> MKNAIVIGAGIGGLAAALRLRHQGYSVTIFEKNDYAGGKLHAIEKDGYRFDLGPSLFTLPHLVENLFALFPEEIIDFGYKSKAISFHYFWDDGTLFKASTDSSQFIEDASKVFKEEKSTIKKYLAKSKSKYELTKSLFLEKSLHKATTYFSLDTVKAIVHAPFLGLNNTLNDENSKF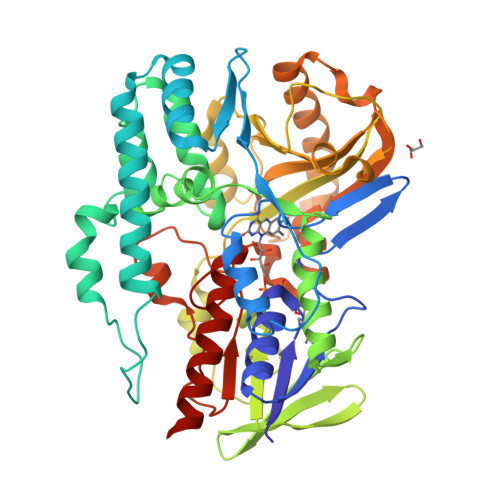KNPKLTQLFNRYATYNGSSPYQTPGIMTMIPHLELGLGTYYPDGGMHRISQSLFELAQKVGVKFRFRESVTNITTSKNKVTGVETKNGSYLSDLVVSNMDIVPTYRNLMKDVPAPEKTLSQERSSSALIFYWGIDREFPELDLHNILFSEDYKTEFEHIFEHKTLAQDPTVYINITSKESSNDAPAGHENWFVMINAPGDYGQDWEQLVEESKKQIIAKIKKCLHVDISKHITTEYILTPQGIEKNTSSYRGALYGAASNNKFAAFLRHPNFNGKIKNLYHVGGSVHPGGGIPLCLLSAQITADLIQKEQLEHHHHHH> MGSDKIHHHHHHM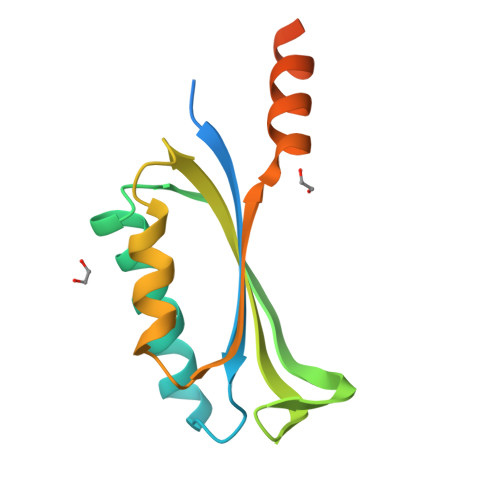AYVKERIYESMFIIAPNVPEEERENLVERVKKIIEERVKGKIDKVERMGMRKFAYEIKKFNEGDYTVIYFRCDGQNLQELENFYRVTPEIIRWQTFRRFDLEKKERKAQREKAAAEATESSEGGSED>GSHMPPN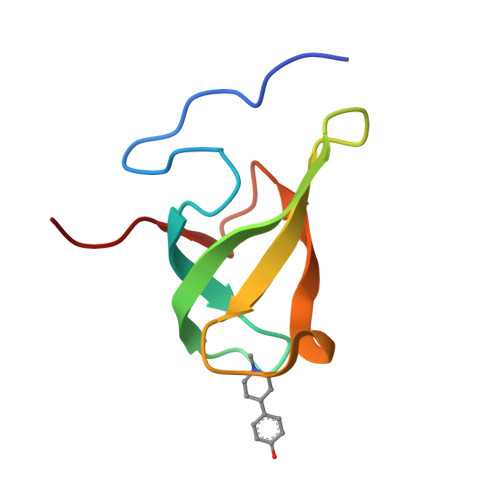RPGITFEIGARLEALDYLQKWYPSRIEKIDYEEGKMLVHFERWSHRYDEWIYWDSNRLRPLER[4x]> MADTQYILPNDIGVSSLDCREAFRLLSPTERLYAYHLSRAAWYGGLAVLLQTSPEAPYIYALLSRLFRAQDPDQLRQHALAEGLTEEEYQAFLVYAAGVYSNMGNYKSFGDTKFVPNLPKEKLERVILGSEAAQQHPEEVRGLWQTCGELMFSLEPRLRHLGLGKEGITTYFSG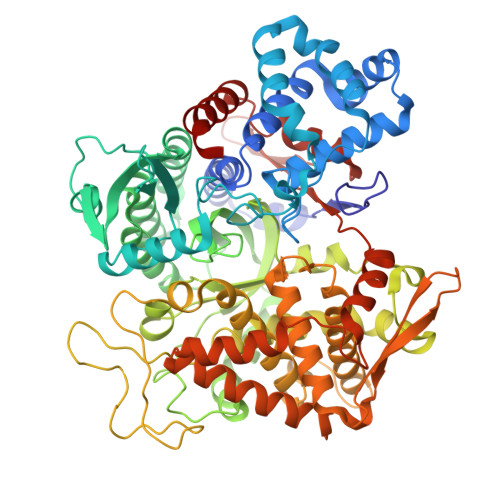NCTMEDAKLAQDFLDSQNLSAYNTRLFKEVDGEGKPYYEVRLASVLGSEPSLDSEVTSKLKSYEFRGSPFQVTRGDYAPILQKVVEQLEKAKAYAANSHQGQMLAQYIESFTQGSIEAHKRGSRFWIQDKGPIVESYIGFIESYRDPFGSRGEFEGFVAVVNKAMSAKFERLVASAEQLLKELPWPPTFEKDKFLTPDFTSLDVLTFAGSGIPAGINIPNYDDLRQTEGFKNVSLGNVLAVAYATQREKLTFLEEDDKDLYILWKGPSFDVQVGLHALLGHGSGKLFVQDEKGAFNFDQETVINPETGEQIQSWYRSGETWDSKFSTIASSYEECRAESVGLYLCLHPQVLEIFGFEGADAEDVIYVNWLNMVRAGLLALEFYTPEAFNWRQAHMQARFVILRVLLEAGEGLVTITPTTGSDGRPDARVRLDRSKIRSVGKPALERFLRRLQVLKSTGDVAGGRALYEGYATVTDAPPECFLTLRDTVLLRKESRKLIVQPNTRLEGSDVQLLEYEASAAGLIRSFSERFPEDGPELEEILTQLATADARFW> MNARSTGQHPARYPGAAAGEPTLDSWQEPPHNRWAFAHLGEMVPSAAVS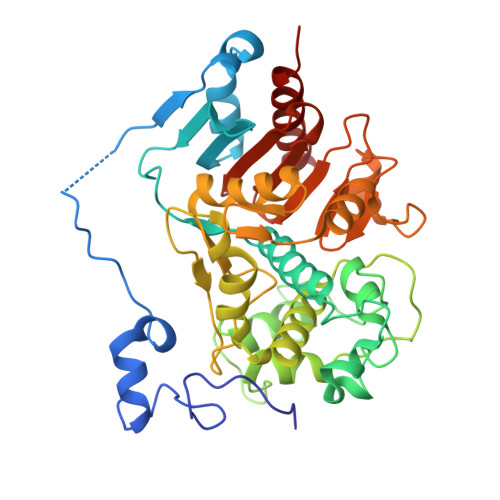RRPVNAPGHALARLGAIAAQLPDLEQRLEQTYTDAFLVLRGTEVVAEYYRAGFAPDDRHLLMSVSKSLCGTVVGALVDEGRIDPAQPVTEYVPELAGSVYDGPSVLQVLDMQISIDYNEDYVDPASEVQTHDRSAGWRTRRHGDPADTYEFLTTLRGDGSTGEFQYCSANTDVLAWIVERVTGLRYVEALSTYLWAKLDADRDATITVDTTGFGFANGGVSCTARDLARVGRMMLDGGVAPGGRVVSEDWVRRVLAGGSHEAMTDKGFTNTFPDGSYTRQWWCTGNERGNVSGIGIHGQNLWLDPLTDSVIVKLSSWPDPDTEHWHRLQNGILLDVSRALDAV>[2x]KHSLPDLPYDYGALEPHINAQIMQLHHSKHHAAYVNNLNVTEEKYQEALAKGDVTAQIA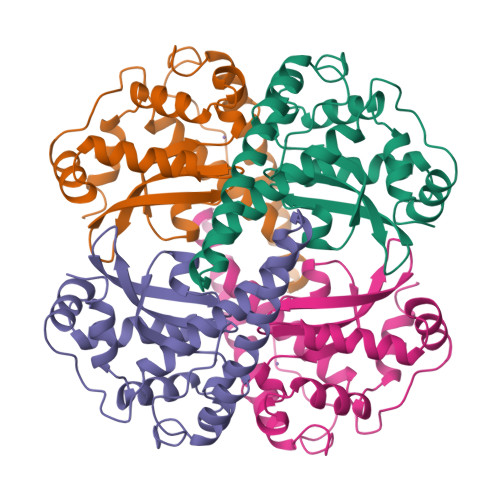LQPALKFNGGGHINHSIFWTNLSPNGGGEPKGELLEAIKRDFGSFDKFKEKLTAASVGVQGSGWGWLGFNKERGHLQIAACPNNDPLQGTTGLIPLLGIDVWEHAYYLQYKNVRPDYLKAIWNVINWENVTERYMACKK CydDC is a prokaryotic ATP-binding cassette (ABC) transporter required for heme assembling in respiratory cytochrome bd oxidase, a promising target for drug discovery. In our structures, CydC and CydD form a heterodimer with each subunit composed of one transmembrane domain (TMD) and one nucleotide-binding domain (NBD). TM4 and TM5 of one subunit associate with TM1-3 and TM6 of another to form a helix bundle in a “domain swapping” manner. The overall fold of CydDC belongs to the type IV family of ABC transporters, commonly known as exporters.

The TM1 of MsCydD is short and the Elbow Helix (EH) is missing while the EH of EcCydD is longer than that of CydC and other type IV ABC transporters. Superposition of TMDs in apo MsCydDC shows that the conformation of TM4 is highly bent in CydD. In the apo structure of MsCydDC, there is a “lateral gate” formed between TM4D and TM6D near the cytoplasmic side. The distance between the bending points of the two helices is 17.3 Å. Thus, it is wide enough to let heme pass through. However, MsCydD lacks the whole EH and the gate is largely open in the apo structure. In the heme-loading structure, the two axial His residues are 4.8 Å away from each other, which is perfect to clamp the iron ion. However, in the apo state structure, the corresponding His residues are 6.8 Å apart and they can no longer coordinate to the iron center. (ii) It enters the inward-open apo state of CydDC through the wide-open lateral gate between TM4D and TM6D.

>[2x]VPLLRHDPLLRLTLELLRPRLGRFLLAAALGVLSLGSALALAGISAWLITRAWQMPPVLDLTVAVVAVRALGISRGVLGYCQRLASHDSALRAAANARTGLYRKLADAPPDEAMRLPSGELVARLGPAVDELADVLVRALLPIVVAVVLGCAAVGVIAVISPASAAVLAVCLVVAGVVAPALAARAAHASETVAAEHRSQRDTAGMLALEHAPELRVSGRLDSVIATFERHHRAWGEAADRAAAPAAVAAAMPTAAMGVSVVGAVIAGIALAPTVAPTTAAILMLLPLSAFEATTALPDAAAQLMRSRVAARRLLELTTPTPLRSRPDVATVDLAPGDRLAVVGPSGSGKTTMLMAIADRLNGAGGETPQRAAVFAEDAHLFDTTVRDNLLVVRGDATDTELVAALDRVGLGEWLAGLPDGLSTVLVGGAAAVSAGQRRRLLIARALISAFPVVLLDEPTENLDAGDARQMLEGLLTPGALFAADRTVVVATHHLPPGFDCPIVRCTGRLAVAGRYLGGIKAFDYKDDDDK;>[2x]SYFQSNVVIAGCTIASAVVLAHIVAGIITNPATALGGETDWAPGLVALAVLWSVRVVAQWFQGRLSQRGATAVIGELSRQVLSSVTTSSPRRLAADRDSAAAVVTRGLDGLRPYFTGYLPAVVLAGILTPAALVVMAAYDWQAAAIVVIALPLIPIFMVLIGLLTAERSAAALTAMTTLQGRMLDLIAGIPTLRAVGRAGGSVQRIAELSASHRRSTMATLRISFLSALVLELLATLGVALVAVSVGLRLVFGDMTLAAGLTALLLAPEVFWPLRRVGAAFHAAQDGKTAAEQALRLCAEPHPPTGHEVVPAGAPVIEVPALKAVMEPGRVTVLTGPNGVGKSTLLQAILGLQESPCGPILVAGVEVGALDRSAWWGRLAWMPHRPVLVPGTVRENLELLGPVPGLDEVCRSVGFDEVLGELPDGSETPLGRGGVGLSLGQRQRLGLVRALGAPADVLLLDEPTAHLDGALEDRVLAAIVARARAGATVVMVGHRAPVLAAADHVVTMESSLVAP>[2x]MRMTWNFHQYYTNRNDGLMGKLVLTDEEKNNLKALRKIIRLRTRDVFEEAKGIAKAVKKSALTFEIIQEKVSTTQIKHLSDSEQREVAKLIYEMDDDARDEFLGLTPRFWTQGSFQYDTLNRPFQPGQEMDIDDGTYMPMPIFESEPKIGHSLLILLVDASLKSLVAEN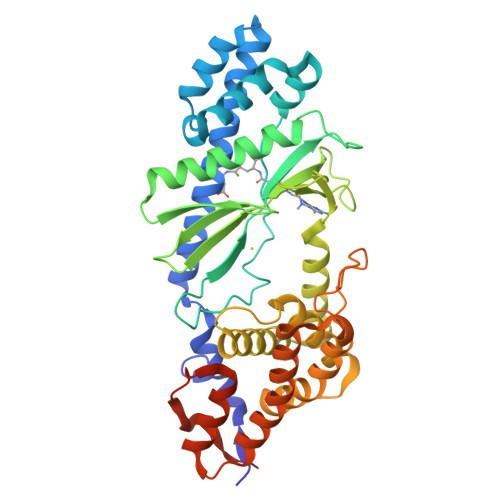HGWKFEAKQTCGRIKIEAEKTHIDVPMYAIPKDELDSENVNLALREGDRKWINSDPKIVEDWFNDSCIRIGKHLRKVCRFMKAWRDAQWDVGGPSSISLMAATVNILDSVAHDASDLGETMKIIAKHLPSEFARGVESPDSTDEKPLFPPSYKHGPREMDIMSKLERLPEILSSAESADSKSEALKKINMAFGNRVTNSELIVLAKALPAFAQELEHHHHHH His domain protein tyrosine phosphatase (HD-PTP/PTPN23) is a tumor suppressor that regulates mitogenic receptor downregulation, endocytic recycling, and cell migration (Chen et al., 2012, Doyotte et al., 2008, Kharitidi et al., 2015, Lee et al., 2007, Ma et al., 2015, Manteghi et al., 2016). A central feature of HD-PTP function is the ability of its Bro1 domain to recruit CHMP4, the major subunit of the ESCRT-III membrane remodeling protein complex (Doyotte et al., 2008, Ichioka et al., 2007, Parkinson et al., 2015). Crystallographic structures of the HD-PTPBro1 domain in complex with the relevant binding regions of SARA, endofin, and all three human CHMP4 isoforms reveal that SARA and endofin binding is similar to that of CHMP4 at the conserved site, but critically extends into a neighboring specific pocket unique to HD-PTP. Altogether, this study identifies the Bro1 domain of HD-PTP as a highly selective interaction hub that coordinates recruitment of endosomal signaling adaptors versus MVB sorting and receptor degradation.

Next, peptides designed from the C-terminal 18–20 residues of CHMP4A, CHMP4B, and CHMP4C were evaluated for binding to HD-PTPBro1. Interestingly, CHMP4 peptides showed much lower affinity to HD-PTPBro1 compared with the SARA/endofin peptides, with KD values of 132 ± 7 μM for CHMP4A, 85 ± 2 μM for CHMP4B, and 89 ± 1 μM for CHMP4C. For the CHMP4 peptides only 11 residues are clearly visible in the electron density maps, whereas 20 residues are visible for the SARA and endofin peptides. All three CHMP4 peptides bind in the same way across helices H5, H6, and H7 of HD-PTPBro1, and form similar van der Waals contacts with a number of conserved residues, including the critical L202/I206 pair. The main CHMP4 anchoring residues are a Leu and a Trp present in all three isoforms (L217 and W220 in CHMP4A and CHMP4B, L228/W231 in CHMP4C), which contact HD-PTPBro1 residues L189, L202, and I206 from two hydrophobic pockets between H5 and H6 and H6 and H7. The mode of binding of CHMP4 peptides to HD-PTPBro1 is similar to that reported for the complexes of CHMP4 peptides with Alix or Brox Bro1 domains (McCullough et al., 2008, Mu et al., 2012). Thus, binding of CHMP4A/B/C to HD-PTPBro1 requires rearrangement of these side chains to accommodate the critical CHMP4 Leu and Trp residues. Overall, the SARA/endofin peptides form an extensive binding interface that encompasses both the CHMP4 site and the S site, resulting in accessible buried surface in HD-PTPBro1 ranging from 762 to 780 Å2, compared with 468 to 473 Å2 for the CHMP4 peptides.

>MEAVPRMPMIWLDLKEAGDFHFQPAVKKFVLKNYGENPEAYNEELKKLELLRQNAVRVPRDFEGCSVLRKYLGQLHYLQSRVPMGSGQEAAVPVTWTEIFSGKSVAHEDIKYEQACILYNLGALHSMLGAMDKRVSEEGMKVSCTHFQCAAGAFAYLREHFPQAYSVDMSRQILTLNVNLMLGQAQECLLEKSMLDNRKSFLVARISAQVVDYYKEACRALENPDTASLLGRIQKDWKKLVQMKIYYFAAVAHLHMGKQAEEQQKFGERVAYFQSALDKLNEAIKLAKGQPDTVQDALRFTMDVIGGKYNSAKKDNDFIYHEAVPALDTLQPVKGAPLVKPLPVNPTDPAVTGPDIFAKLV[4x];>[4x]PKVDEDEEALKQLAEWVS> MKTIT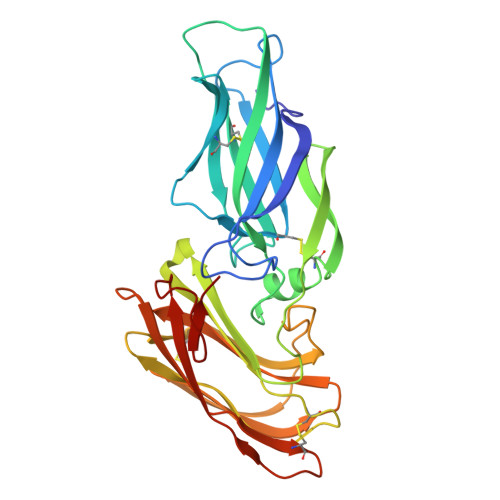GVFNSFDSLTWTRSVEYVYKGPETPTWNAVLGWSLNSTTADPGDTFTLILPCVFKFITTQTSVDLTADGVSYATCDFNAGEEFTTFSSLSCTVNSVSVSYARVSGTVKLPITFNVGGTGSSVDLADSKCFTAGKNTVTFMDGDTKISTTVDFDASPVSPSGYITSSRIIPSLNKLSSLFVVPQCENGYTSGIMGFVASNGATIDCSNVNIGISKGLNDWNFPVSSESFSYTKTCTSTSITVEFQNVPAGYRPFVDAYISAENIDKYTLTYANEYTCENGNTVVDPFTLTWWWYKNSEADSDGDVIVV>GSHMGSGQVTLDFFQFKAEAADWFKQAAQEFEKENPDIRININNSANAQTDLRTRFVKDRVPDVITFNGDYSFGTFAASGVFHDFTDDPLVSELNEGMVNIAKNLVQTSDPAKKRLYGLPFAGNASGYIYNKDLFRKVGLDPDNPPQTWDEFIAMLKKFRDAGINPVQATLADAWTTQAPLASLAGTLVPESEYAALKSGDTTFKQIWTEPIEKEIELFKYADSEKGVTYQQGTQNFAKGTAAIIPLGTYAIPQITMVNKDIDLGFAQMPATNDASKQILTAGDDVILTMGANSRHKEQSM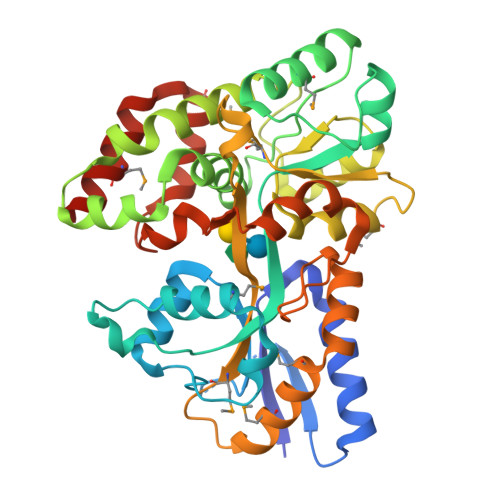RFIRFLMSKKQLENYADAQSAITPLKETYFGNKALEPVRPFFESNRVADFCDHYIPSSINIGGYLQSAIMSGNVNQFIDSMQNEWNKVQARDFRK[2x]> MSDPFDYLF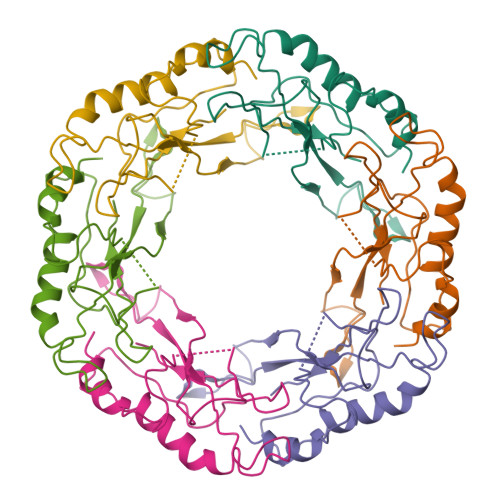LEPLLIERIRSEVPGLAIVSGVPDLATLSEQDQPAPSAYVVYLGDETGTGADHQGGQRAIQTVGQQWAVVLVVHYADSSNSGEGARREAGPLLGRLVKALTGWAPAIDVAPLARSARQSPATYASGYLYFPLVFTARFVYPRIKSWKP Here, we characterize a protein called MamO that helps to initiate the formation of a magnetic mineral called magnetite in cells of the magnetotactic bacterium Magentospirillum magneticum AMB-1. Although predicted to be a trypsin-like protease, we show that MamO has lost its ancestral catalytic activity and instead gained a new function as a metal-binding scaffold. Two genes in the MAI, mamE and mamO, are homologous to the HtrA proteases, a ubiquitous family of trypsin-like enzymes that functions using His-Asp-Ser catalytic triads. It appears to have lost the ability to perform serine protease activity and instead performs two noncatalytic functions: direct metal binding to promote magnetite nucleation and activation of MamE’s proteolytic activity.

To explore this possibility further, we determined the crystal structure of the protease domain. It crystallizes as a monomer with the chymotrypsin fold and the catalytic residues properly placed. Loop L1 of MamO adopts the inactive conformation seen in many HtrA proteases in which the main chain carbonyl of residue 192 (chymotrypsin numbering; W222 in MamO) prevents access to the oxyanion hole. Although glycine is highly conserved at position 193 in the trypsin family and is critical for catalysis, MamO contains a glutamate (E223) at this position. Therefore, the active configuration of MamO would contain a strong steric clash between the E223 side chain and the main chain carbonyl of W222. The active configuration is strongly disfavored unless glycine occupies position 193, indicating that the E223 side-chain in MamO likely prevents the formation of an oxyanion hole. While refining the MamO structure, we observed a peptide bound near the predicted peptide-binding groove. We suspect its source is the flexible N-terminal region from a neighboring MamO in the crystal that is not built into the model. However, the bulky side-chain of W222 in MamO seems to block the exit path between loops LA and LD, forcing the peptide away from the catalytic center. Overall, the structural features of the L1 loop appear incompatible with protease activity: E223 provides an energetic barrier to catalysis while W222 serves as a physical barrier to productive substrate binding.

> LYHTVPPAVVGVGGGGVNAGPVASGAIVGTNGYVITTLHSVSKLPEISVQVATTGGIRRFPAQVVKTIPGHDLALLKMQTTEKFLHFRMADVQTVVPGQQVFAFGRNMAGAPLVRQGLVQSADAPLAVGATQITHLLRSDAVYSWEQTGGPLVNAQGDLVGINIAATGPTGKVEGFTVPAQVIVSHLQD>GAMKVEVITGEEAESNVLQMQCKLFVFDKTSQSWVERGRGLLRLNDMASTDDGTLQSRLVMRTQGSLRLILNTKLWAQMQIDKASEKSIRITAMDTEDQGVKVFLISASSKDTGQLYAALHHRILALRSRVEQEQEAK[4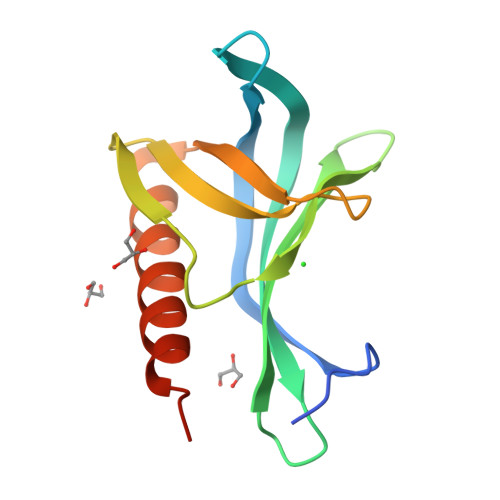x]>[2x]MTTGLSTAGAQDIGRSSVRPYLEECTRRFQEMFDRHVVTRPTKVE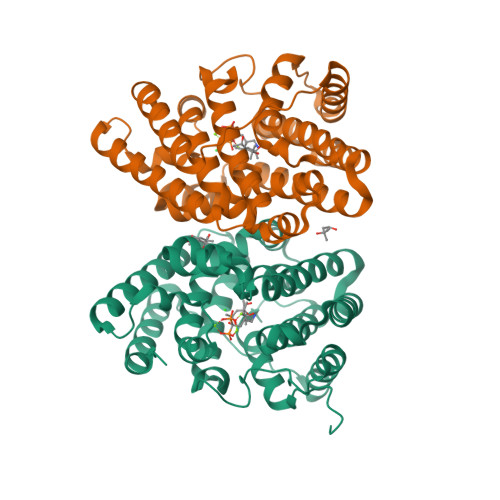LTDAELREVIDDCNAAVAPLGKTVSDERWISYVGVVLWSQSPRHIKDMEAFKAVCVLNCVTFVWDDMDPALHDFGLFLPQLRKICEKYYGPEDAEVAYEAARALVTSDHMFRDSPIKAALCTTSPEQYFRFRVTDIGVDFWMKMSYPIYRHPEFTEHAKTSLAARMTTRGLTIVNDFYSYDREVSLGQITNCFRLCDVSDETAFKEFFQARLDDMIEDIECIKAFDQLTQDVFLDLIYGNFVWTTSNKRYKTAVNDVNSRIQAAALEHHHHHH> MQPPELEIGMPKRHREHIRKNLNILVEWTNYERLAMECVQQGILTVQMLRNTQDLNGKPFNMDEKDVRVEQHRRLLLKITQRGPTAYNLLINALRNINCLDAAVLLESVDESDSRPPFISLNERRTSRKSADIVDTPSPEASEGPCVSKLRNEPLGALTPYVGVVDGPEVKKSKKIHGGDSAILGTYKMQSRFNRGVLLMVNIMDYPDQNRRRIGAEKDSKSLIHLFQELNFTIFPYGNVNQDQFFKLLTMVTSSSYVQNTECFVMVLMTHGNSVEGKEKVEFCDGSVVDMQKIKDHFQTAKCPYLVNKPKVLMFPFCRGDEYDLGHP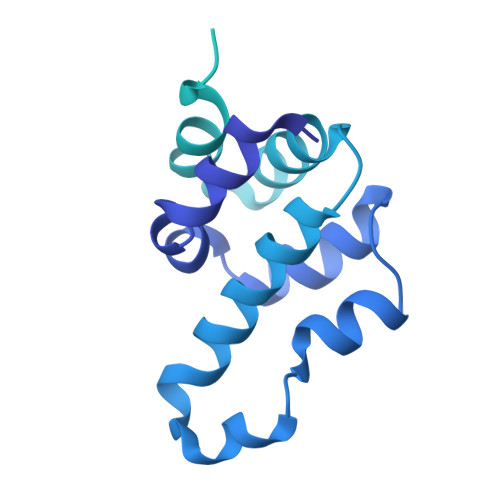KNQGNLMEPVYTAQEEKWPDTQTEGIPSPSTNVPSLADTLVCYANTPGYVTHRDLDTGSWYIQKFCQVMADHAHDTDLEDILKKTSEAVGNKRTKKGSMQTGAYDNLGFNKKLYFNPGFFNE>NCSKIHLSTKLLAVDFPAHFVKSISCQICEHILADPVETSCKHLFCRICILRCLKVMGSYCPSCRYPCFPTDLESPVKSFLNILNSLMVKCPAQDCNEEVSLEKYNHHVSSHKESKETLVHINKGGRPRQHLLSLTRRAQKHRLRELKIQVKEFADKEEGGDVKAVCLTLFLLALRARNEHRQADELEAIMQGRGSGLQPAVCLAIRVNTFLSCSQYHKMYRTVKAITGRQIFQPLHALRNAEKVLLPGYHPFEWQPPLKNVSSRTDVGIIDGLSGLASSVDEYPVDTIAKRFRYDSALVSALMDMEEDILEGMRSQDLDDYLNGPFTVVVKESCDGMGDVSEKHGSGPAVPEKAVRFSFTVMRITIEHGSQNVKVFEEPKPNSELCCKPLCLMLADESDHETLTAILSPLIAEREAMKSSELTLEMGGIPRTFKFIFRGTGYDEKLVREVEGLEASGSVYICTLCDTTRLEASQNLVFHSITRSHAENLQRYEVWRSNPYHESVEELRDRVKGVSAKPFIETVPSIDALHCDIGNAAEFYKIFQLEIGEVYKHPNASKEERKRWQATLDKHLRKRMNLKPIMRMNGNFARKLMTQETVDAVCELIPSEERHEALRELMDLYLKMKPVWRSSCPAKECPESLCQYSFNSQRFAELLSTKFKYRYEGKITNYFHKTLAHVPEIIERDGSIGAWASEGNQSGNKLFRRFRKMNARQSKCYEMEDVLKHHWLYTSKYLQKFMNAHNALKSSGFTMNSKETLGDPLGIEDSLESQDSMEF[2x];>[2x]MSLQMVTVGHNIALIQPGFSLMNFDGQVFFFGQKGWPKRSCPTGVFHFDIKQNHLKLKPAIF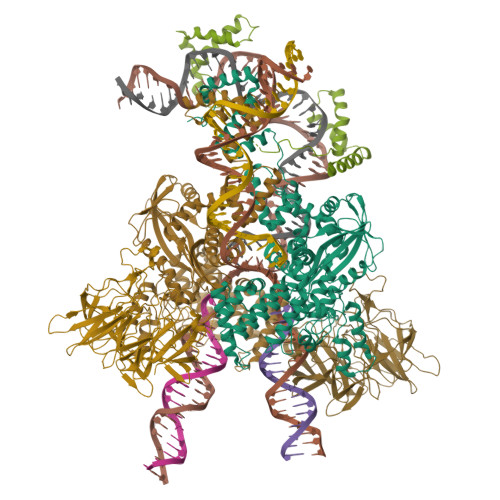SKDSCYLPPLRYPATCSYKGSIDSDKHQYIIHGGKTPNNELSDKIYIMSVACKNNKKVTFRCTEKDLVGDVPEPRYGHSIDVVYSRGKSMGVLFGGRSYMPSTQRTTEKWNSVADCLPHVFLIDFEFGCATSYILPELQDGLSFHVSIARNDTVYILGGHSLASNIRPANLYRIRVDLPLGTPAVNCTVLPGGISVSSAILTQTNNDEFVIVGGYQLENQKRMVCSLVSLGDNTIEISEMETPDWTSDIKHSKIWFGSNMGNGTIFLGIPGDNKQAMSEAFYFYTLRCSEEDLSEDQKIVSNSQTSTEDPGDSTPFEDSEEFCFSAEATSFDGDDEFDTYNEDDEDDESVTGYWITCCPTCDVDINTWVPFYSTELNKPAMIYCSHGDGHWVHAQCMDLEERTLIHLSEGSNKYYCNEHVQIARALQAPKRNPPLQKPPMKSLHKKGSGKVLTPAKKS;> MGKGDPKKPRGKMSSYAFFVQTCREEHKKKHPDASVNFSEFSKKCSERWKTMSAKEKGKFEDMAKADKARYEREMKTYIPPKGETKKKFKDPNAPKRPPSAFFLFCSEYRPKIKGEHPGLSIGDVAKKLGEMWNNTAADDKQPYEKKAAKLKEKYEKDIAAYR>MTTSHGLIESQLSYYRARASEYDATFVPYMDSAAPAALERLRAGNIRGDVLELASGTGYWTRHLSGLADRVTALDGSAEMIAEAGRHGLDNVEFRQQDLFDWTPDRQWDAVFFAHWLAHVPDDRFEAFWESVRSAVAPGGVVEFVDVTDHERRLEQQDDSEPEVAVRRTLQDGRSFRIVKVFRSPAELTERLTALGWSCSVDEVHPGFLYATCRP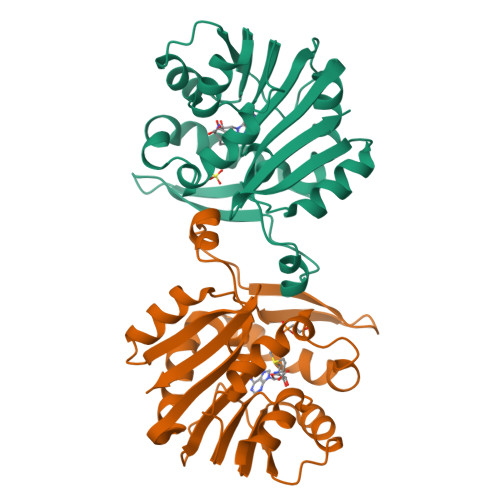GPR[4x]> GIDPFTEEEIRMELSPDLISACLALEKYLDNPNALTERELKVAYTTVLQEWLRLACRSDAHPELVRRHLVTFRAMSARLLDYVVNIADSNGNTVLHYSVSHANFPVVQQLLDSGVCKVDKQNRAGYSPIMLTALATLKTQDDIETVLQLFRLGNINAKASQAGQ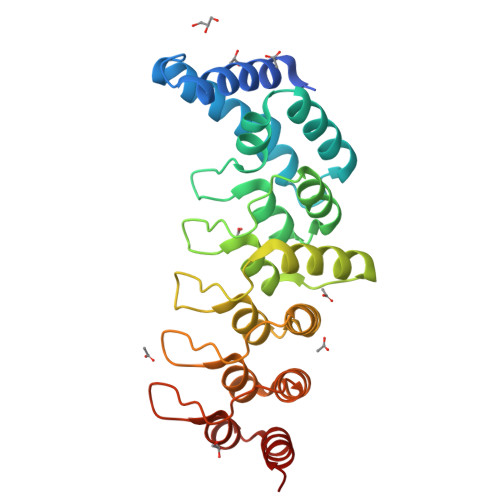TALMLAVSHGRVDVVKALLACEADVNVQDDDGSTALMCACEHGHKEIAGLLLAVPSCDISLTDRDGSTALMVALDAGQSEIASMLYSRMNIK>SMEILQ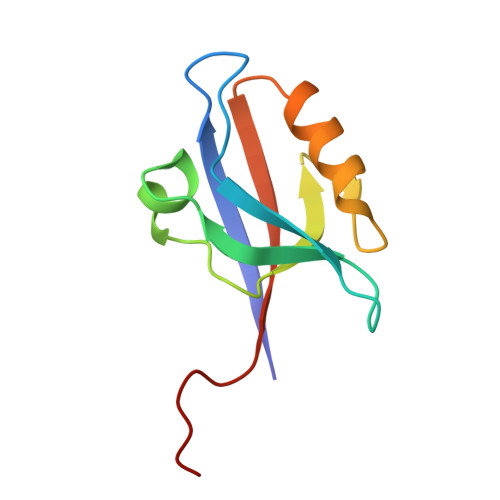VALHKRDSGEQLGIKLVRRTDEPGVFILDLLEGGLAAQDGRLSSNDRVLAINGHDLKYGTPELAAQIIQASGERVNLTIARPGKPEIEL[2x]>GPSDMYVHVGNLIYRNLHLFNSEMHESILVSYSSDLIIYRTNTVGDDYIPSCDCTQA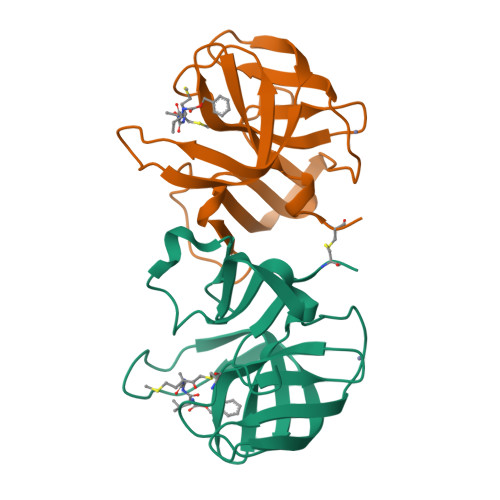TYYCKHKNRYFPITVTSHDWYEIQESEYYPKHIQYNLLIGEGPCEPGDCGGKLLCKHGVIGIVTAGGDNHVAFIDLRHFHCAEEQ[2x]> MPKTISVRVTTMDAELEFAIQPNTTGKQLFDQVVKTIGLREVWFFGLQYQDTKGFSTWLKLNKKVTAQDVRKESPLLFKFRAKFYPEDVSEELIQDITQRLFFLQVKEGILNDDIYCPPETAVLLASYAVQSKYGDFNKEVHKSGYLAGDKLLPQRVLEQHKLNKDQWEERIQVWHEEHRGMLREDAV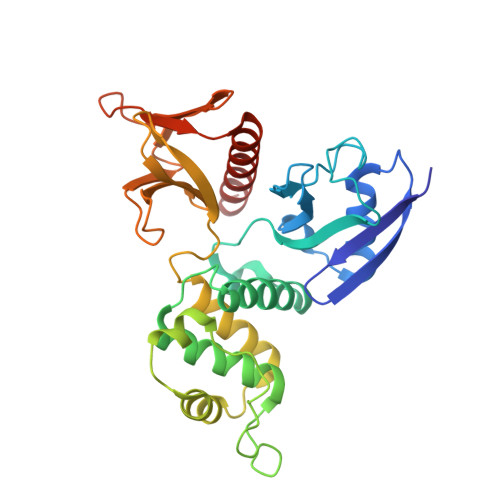LEYLKIAQDLEMYGVNYFSIKNKKGSELWLGVDALGLNIYEQNDRLTPKIGFPWSEIRNISFNDKKFVIKPIDKKAPDFVFYAPRLRINKRILALCMGNHELYMRRRK> MISDSMTVEEIRLHLGLALKEKDFVVDKTGVKTIEIIGASFVADEPFIFGALNDEYIQRELEWYKSKSLFVKDIPGETPKIWQQVASSKGEINSNYGWAIWSEDNYAQYDMCLAELGQNPDSRRGIMIYTRPSMQFDYNKDGMSDFMCTNTVQYLIRDKKINAVVNMRSNDVVFGFRNNYAWQKYVLDKLVSDLNAGDSTRQYKAGSIIWNVGSLHVYSRHFYLVDHWWKTGETHISKKDYVGKYALEHHHHHHHH

Herein, we described the XFEL structure of dCMP hydroxymethylase (dCH) from bacteriophage T4 (T4dCH) at 1.9-Å resolution using the Pohang Accelerator Laboratory (PAL) XFEL. The dCH is the first identified viral enzyme from T-even phage, and it gives viral phage the opportunity to escape the restriction-modification system of host bacteria by the hydroxymethylation of a cytosine base. It belongs to the thymidylate synthase (TS) superfamily and catalyzes dCMP to hydroxymethyl-dCMP (hmdCMP) using 5,10-methylenetetrahydrofolate (5,10-mTHF) and water as a methyl and hydroxyl donor, respectively. However, questions about the cytosine modification catalysis remain to be answered because the methylene intermediate structure has not been elucidated yet.

After processing the entire dataset with a completeness of 100%, we solved the XFEL structure of T4dCH D179N at a resolution of 1.9 Å. Intriguingly, a bulky difference map was detected in the substrate binding site of the XFEL structure even though no substrate-like compounds were added during the purification and crystallization steps. A fragment spectrum of m/z ratio 321.0495 in D179N was detected at the same positions of the dTMP fragments. Therefore, by combining XFEL crystallography and mass spectrometric analysis, the unknown substance bound to T4dCH D179N was revealed as a dTMP molecule. The phosphate moiety of dTMP was recognized by the side chain atoms of Lys28, Arg168, Ser169, Arg123′, Arg124′, and a water molecule (Wat603), which formed a hydrogen bond with the main-chain atom of Phe146. For the recognition of the thymine base, the carbonyl oxygen at position 2 was recognized by the side-chain nitrogen atom of Asn170 and the main-chain nitrogen atom of Asp171, and the carbonyl oxygen at position 4 was recognized by the side-chain oxygen atom of Tyr96 and side-chain nitrogen atom of Asn179. Interestingly, the Asn residue of the mutant recognized the N3 atom and the carbonyl oxygen at position 4 in the thymine base, whereas the carboxylate of Asp179 of WT interacted with the N3 atom and primary amine group at position 4 of the cytosine base; this is shown in the binary complex structure. In comparison with the ligand geometry of dCMP in the binary complex of T4dCH WT, the ligand geometry of dTMP in the XFEL structure of D179N exhibited a critical difference around a methyl group at the C5 position in the pyrimidine base. Our dTMP-bound structure well mimicked the methylene intermediate that was the methylated pyrimidine nucleotide complex. We carefully explored the XFEL structure and found that this electron density matches with the sodium ion that forms an octahedral geometry with the main chain oxygen atoms of Lys72, Ile74, and Gly76, and side chain hydroxyl group of Thr78, in addition to two water molecules.>LTFESTSRFAEVDVDGPLKLHYHEAGVGNDQTVVLLHGGGPGAAS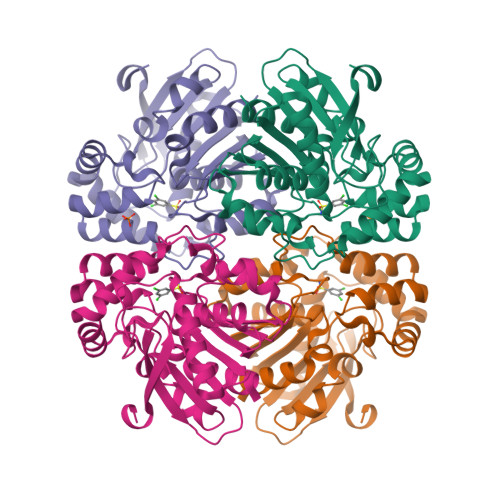WTNFSRNIAVLARHFHVLAVDQPGYGHSDKRAEHGQFNRYAAMALKGLFDQLGLGRVPLVGNSLGGGTAVRFALDYPARAGRLVLMGPGGLSINLFAPDPTEGVKRLSKFSVAPTRENLEAFLRVMVYDKNLITPELVDQRFALASTPESLTATRAMGKSFAGADFEAGMMWREVYRLRQPVLLIWGREDRVNPLDGALVALKTIPRAQLHVFGQCGHWVQVEKFDEFNKLTIEFLG[2x]>HHHHHHENLYFQGAASMLADSFEQEASREVDASKGLTNSETLQVEQDGKVRLSHQVRHQVALPPNYDYTPIAEHKRVNEARTYPFTLDPFQDTAISCIDRGESVLVSAHTSAGKTVVAEYAIAQSLKNKQRVIYTSPIKALSNQKYRELLAEFGDVGLMTGDITINPDAGCLVMTTEILRSMLYRGSEVMREVAWVIFDEVHYMRDKERGVVWEETIILLPDKVRYVFLSATIPNAMEFAEWICKIHSQPCHIVYTNFRPTPLQHYLFPAHGDGIYLVVDEKSTFREENFQKAMASISNQIGDDPNSTDSRGKKGQTYKGGSAKGDAKGDIYKIVKMIWKKKYNPVIVFSFSKRDCEELALKMSKLDFNSDDEKEALTKIFNNAIALLPETDRELPQIKHILPLLRRGIGIHHSGLLPILKEVIEILFQEGFLKVLFATETFSIGLNMPAKTVVFTSVRKWDGQQFRWVSGGEYIQMSGRAGRRGLDDRGIVIMMIDEKMEPQVAKGMVKGQADRLDSAFHLGYNMILNLMRVEGISPEFMLEHSFFQFQNVISVPVMEKKLAELKKDFDGIEVEDEENVKEYHEIEQAIKGYREDVRQVVTHPANALSFLQPGRLVEISVNGKDNYGWGAVVDFAKRINKRNPSAVYTDHESYIVNVVVNTMYIDSPVNLLKPFNPTLPEGIRPAEEGEKSIC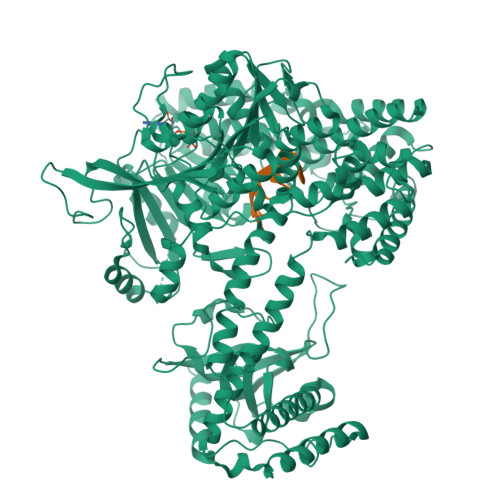AVIPITLDSIKSIGNLRLYMPKDIRASGQKETVGKSLREVNRRFPDGIPVLDPVKNMKIEDEDFLKLMKKIDVLNTKLSSNPLTNSMRLEELYGKYSRKHDLHEDMKQLKRKISESQAVIQLDDLRRRKRVLRRLGFCTPNDIIELKGRVACEISSGDELLLTELIFNGNFNELKPEQAAALLSCFAFQERCKEAPRLKPELAEPLKAMREIAAKIAKIMKDSKIEVVEKDYVESFRHELMEVVYEWCRGATFTQICKMTDVYEGSLIRMFKRLEELVKELVDVANTIGNSSLKEKMEAVLKLIHRDIVSAGSLYL[2x]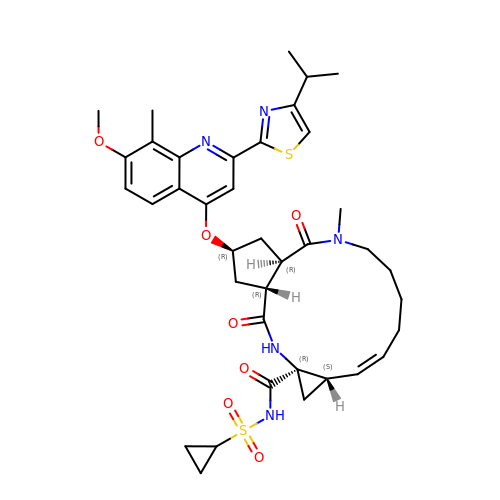(2R,3aR,10Z,11aS,12aR,14aR)-N-(cyclopropylsulfonyl)-2-({7-methoxy-8-methyl-2-[4-(1-methylethyl)-1,3-thiazol-2-yl]quinolin-4-yl}oxy)-5-methyl-4,14-dioxo-2,3,3a,4,5,6,7,8,9,11a,12,13,14,14a-tetradecahydrocyclopenta[c]cyclopropa[g][1,6]diazacyclotetradecine-12a(1H)-carboxamide | C38 H47 N5 O7 S2 | JTZZSQYMACOLNN-VDWJNHBNSA-N> MSVNQKEIEIAIEYFKNYISVGEIV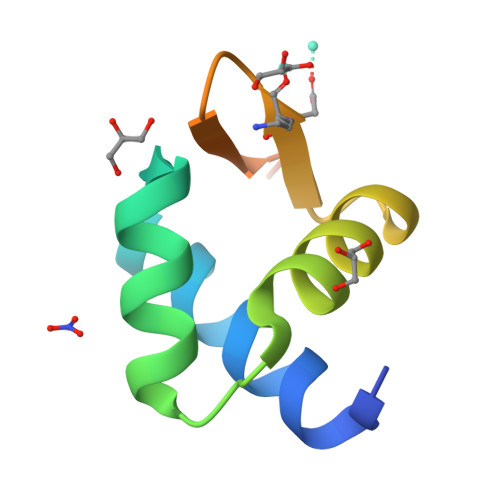ATMDLKARGISNPQAVISKLIEMGIIEKGEGCYNLVRKSTDKKLEHHHHHH>MASDAQAGPAPSRDDRVDRQPRLPAAPRVAEVGLNAPSVDYPFQWVVASYDGSEAKNLSDDLSGSATLTKVMANYRHAELTSVELEVCPLAAAFSKPISVSAVWTIASISPASASETSYYGGRLFTVGGPVLMSSTTHLPADLTRLNPVLKGPVK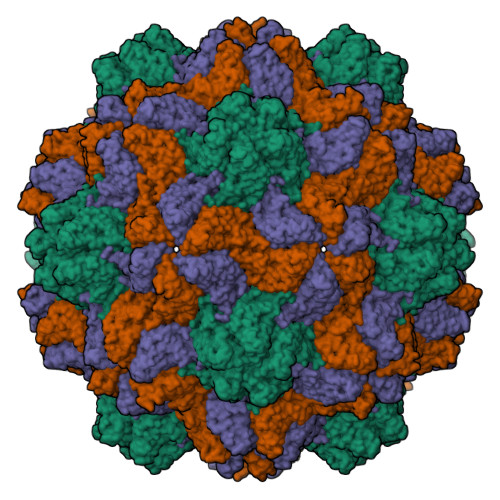YTDCPRFSYSVYSNGGTKGTNLCTIILRGVVRLSGPSGNLLA[3x]>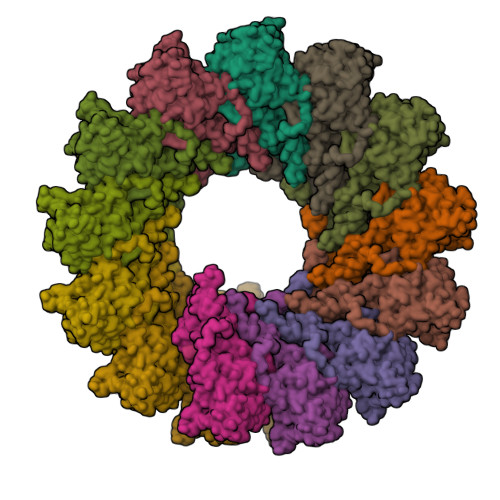 GMATLLRSLALFKRNKDRTPLTAGSGGAIRGIKHVIVVPVPGDSSIVTRSRLLDRLVRLAGDPYISGPKLTGVMISILSLFVESPSQLIQRITDDPDVSIRLVEVIQSEKSLSGLTFASRGANMEDEADDYFSIQAGEEGDTRGTHWFENKEIVEIEVQDPEEFNILLASILAQIWILLAKAVTAPDTAADSETRRWIKYTQQRRVVGEFRLDKGWLDAVRNRIAEDLSLRRFMVALILDIKRTPGNKPRIAEMICDIDTYIVEAGLASFILTIKFGIETMYPALGLHEFSGELTTVESLMNLYQQMGETAPYMVILENSIQNKFSAGSYPLLWSYAMGVGVELENSMGGLNFGRSYFDPAYFRLGQEMVRRSAGKVSSSLAAELGITAEDAKLVSEIAAQANDDRVEHHHHHHHH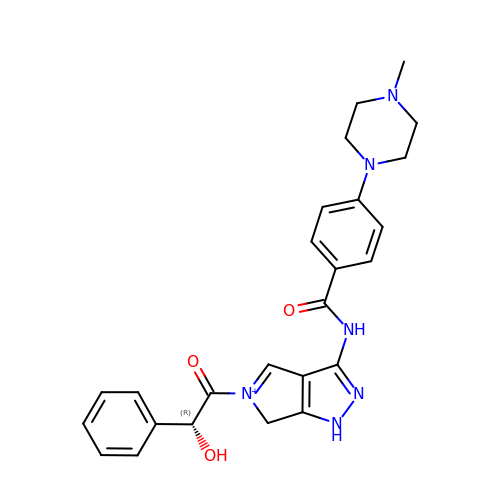5-[(2R)-2-hydroxy-2-phenylacetyl]-3-({[4-(4-methylpiperazin-1-yl)phenyl]carbonyl}amino)-1,6-dihydropyrrolo[3,4-c]pyrazol-5-ium  | C25 H27 N6 O3 | FCLFBDYOCRVSHV-JOCHJYFZSA-O> MSELIVNVINGPNLGRLGRREPAVYGGTTHDELVALIEREAAELGLKAVVRQSDSEAQLLDWIHQAADAAEPVILNAGGLTHTSVALRDACAELSAPLIEVHISNVHAREEFRRHSYLSPIATGVIVGLGIQGYLLA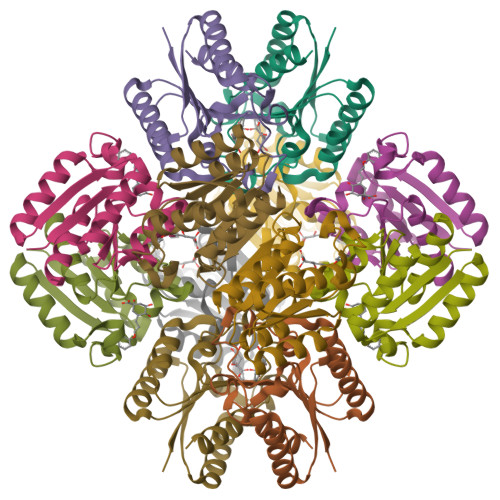LRYLAEHVGT> HTLVWGVWVNGVDQGDGRNIYIRSPPNNNPVKNLTSPDMTCNVDNRVVPKSVPVNAGDTLTFEWYHNTRDDDIIASSHHGPIAVYIAPAASNGQGNVWVKLFEDAYNVTNSTWAVDRLITAHGQHSVVVPHVAPGDYLFRAEIIALHEADSLYSQNPIRGAQFYISCAQITINSSDDSTPLPAGVPFPGAYTDSTPGIQFNIYTTPATSYVAPPPSVWSGALGGSIAQVGDASLE

Lytic polysaccharide monooxygenases (LPMOs) are copper metalloenzymes which cleave polysaccharides oxidatively and are important in pathogen biology, carbon cycling and biotechnology. The Lentinus similis family AA9 isoform A (LsAA9_A) has been extensively studied as a model system because its activity towards smaller soluble saccharide substrates has allowed detailed structural characterization of its interaction with a variety of substrates by X-ray crystallography at high resolution. Fungal LPMOs are some of many enzymes secreted by fungi to break down plant matter, namely cellulose, and release glucose. LPMOs randomly oxidize recalcitrant crystalline cellulose, disrupting local crystallinity and creating new cellodextrin chain ends that serve as additional starting points for the endo- and exo-activities of glycoside hydrolases (GHs; Agger et al., 2014).

Here, the joint X-ray/neutron room-temperature crystallographic structure of carbohydrate-free LsAA9_A in the copper(II) resting state refined against X-ray and neutron data at 2.1 and 2.8 Å resolution, respectively, is presented. No residual F o − F c electron density was observed for an alternate conformation of His78 flipped away from the active-site Cu2+. However, residual F o − F c electron density indicated that a Cl− ion from the crystallization condition alternatively coordinates the Cu2+ ion instead of His78 as observed in the structure of LsAA9_A previously solved at pH 3.5. The occupancies of His78 and Cl− refined to 0.75 and 0.25, respectively. The N-terminal amino group is neutral. The distances from H2O-eq and H2O-ax to Cu2+ are 2.1 and 2.7 Å, respectively, confirming that the copper ion is in the resting oxidation state, copper(II), and validating the use of the X-ray data for joint refinement. In the structure presented here, Tyr164 is positioned in the axial position of the copper with a Cu–OTyr distance of 2.80 Å. The Tyr164 OH group forms a hydrogen bond to the side-chain carbonyl group of Gln162 with an OTyr164–OGln162 distance of 2.72 Å.> MTMDFSDPDMEFLCLTRQKLMEATSIPFDGKKNCWVPDPDFGFVGAEIQSTKGDEVTVKTDKTQETRVVKKDDIGQRNPPKFEMNMDMANLTFLNEASILHNLRSRYESGFIYTYSGLFCIAINPYRRLPIYTQGLVDKYRGKRRAEMPPHLFSIADNAYQYMLQDRENQSMLITGESGAGKTENTKKVIQYFALVAASLAGKKDKKEEEKKKDEKKGTLEDQIVQCNPVLEAYGNAKTTRNNNSSRFGKFIRIHFGTQGKIAGADIETYLLEKSRVTYQQSAERNYHIFYQLLSPAFPENIEKILAVPDPGLYGFINQGTLTVDGIDDEEEMGLTDTAFDVLGFTDEEKLSMYKCTGCILHLGEMKWKQRGEQAEADGTAEAEKVAFLLGVNAGDLLKCLLKPKIKVGTEYVTQGRNKDQVTNSIAALAKSLYDRMFNWLVRRVNQTLDTKAKRQFFIGVLDIAGFEIFDFNSFEQLCINYTNERLQQFFNHHMFVLEQEEYKKEGIVWEFIDFGLDLQACIELIEKPMGILSILEEECMFPKASDTSFKNKLYDNHLGKNPMFGKPKPPKAGCAEAHFCLHHYAGSVSYSIAGWLDKNKDPINENVVELLQNSKEPIVKMLFTPPRILTPGGKKKKGKSAAFQTISSVHKESLNKLMKNLYSTHPHFVRCIIPNELKTPGLIDAALVLHQLRCNGVLEGIRICRKGFPNRIIYSEFKQRYSILAPNAVPSGFADGKVVTDKALSALQLDPNEYRLGNTKVFFKAGVLGMLEDMRDERLSKIISMFQAHIRGYLMRKAYKKLQDQRIGLTLIQRNVRKWLVLR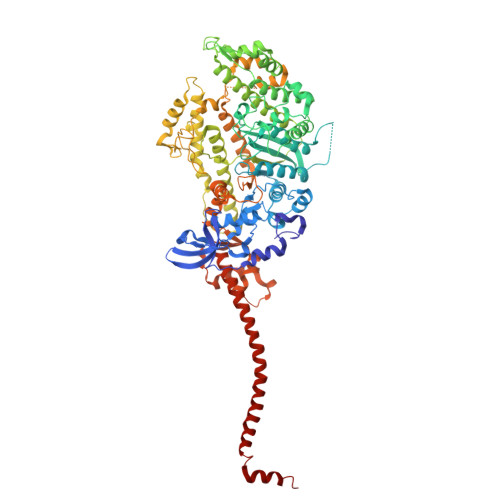NWEWWRLFNKVKPLL>MGNDDIRQVYYRDKGISHAKAGRYSEAVVMLEQVYDADAFDVEVALHLGIAYVKTGAVDRGTELLERSIADAPDNIKVATVLGLTYVQVQKYDLAVPLLVKVAEANPVNFNVRFRLGVALDNLGRFDEAIDSFKIALGLRPNEGKVHRAIAYSYEQMGSHEEALPHFKKANELDERSAVELA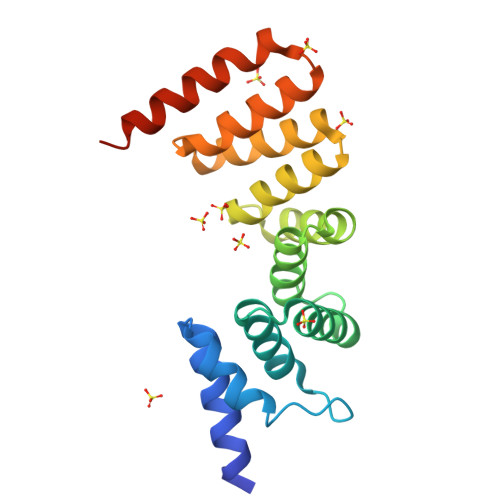LVPR[2x]> MSIVTKSIVNADAEARYLSPGELDRIKAFVTGGAARLRIAETLTGSRETIVKQAG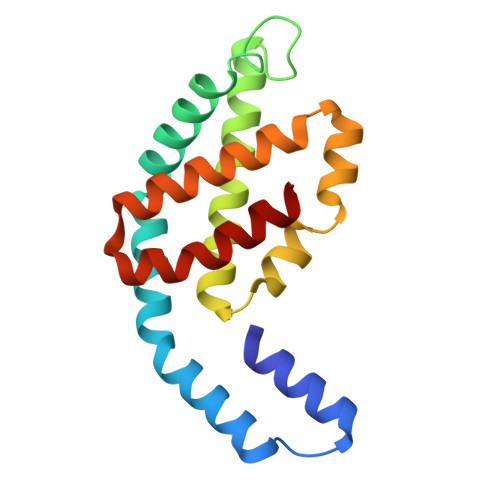DRLFQKRPDIVSPGGNAYGEEMTATCLRDMDYYLRLVTYGVVSGDVTPIEEIGLVGVREMYRSLGTPIEAVAQSVREMKEVASGLMSSDDAAEASAYFDFVIGKMS>MGSSHHHHHHMIRKVLVANRGEIAVRIIRACQELGIRTVVAYSTADRDSLAVRLADEAVCIGPPPAAKSYLNAPALISAALVSGCDAIHPGYGFLSENPYFAEMCADCKLTFIGPPPEPIRLMGDKAIGRETMRKAGVPTVPGSDGEVRSLEEAIDVARQIGYPVLLKPSGGGGGRGMRVAYDEADLQRAFPTARAEAEAAFGNGALLLEKYLTRVRHVEIQVLADQYGHAIHLGERDCSAQRRHQKIVEEAPSPAVTPELRERMGADAVRGIKSIGYVNAGTLEFLLDQDGNYYFIEMNTRIQVEHPVTEQVTGIDLVRWQLLIASGERLTLRQEDIKITRHAIECRINAEDPERDFLPASGEVEFYLPPGGPGVRVDSHLYSGYTPPGTYDSLLAKIITFGDTRDEALNRMRRALNECVITGIKTTIPFQLALIDDPEFRAGRIHTGYVAELLRQWKETLNPV[2x]

Acetyl-CoA carboxylases (ACCs) convert acetyl-CoA to malonyl-CoA, a key step in fatty acid biosynthesis and autotrophic carbon fixation pathways. Three functionally distinct components, biotin carboxylase (BC), biotin carboxyl carrier protein (BCCP), and carboxyltransferase (CT), are either separated or partially fused in different combinations, forming heteromeric ACCs. Here, we identify two BC isoforms (BC1 and BC2) from Chloroflexus aurantiacus, a filamentous anoxygenic phototroph that employs 3-hydroxypropionate (3-HP) bi-cycle rather than Calvin cycle for autotrophic carbon fixation. To investigate the structural basis of BC1 as a bi-functional enzyme, we determined the crystal structures of BC1 and BC2 at 3.2 Å and 3.0 Å resolutions, respectively.

Notably, C. aurantiacus BC1 but not BC2, as well as the BCs from S. coelicolor, Roseiflexus castenholzii, and M. tuberculosis possess a C-terminal biotin/lipoyl attachment domain. Crystal packing analyses revealed two BC1 homodimers, but only one BC2 homodimer in each asymmetric unit. The superposition of one BC1-BC monomer with that of BC2 gave a root mean square deviation (RMSD) value of 0.654 Å, indicating that BC1 and BC2 possessed the same BC architectures. Each BC1-BC and BC2 homodimer was stabilized by extensive hydrogen bonding interactions between conserved amino acid pairs in the N- and C-terminal sub-domains. Specifically, the dimer interface residues Tyr44, Val328, Ser393 in BC1-BC homodimer, and Arg310 in BC2 dimer are not conserved with other reported BCs. Using NaHCO3 and biotin as substrates, both BC1 and BC2 were enzymatically active in catalyzing the biotin carboxylation reactions. However, BC1 had a relatively higher substrate affinity and turnover number than BC2. For BC2 that lacks a fused BCCP domain, it showed relatively lower biotin carboxylase activity and a dimer formation in solution. By contrast, the expression level of BC2 gradually decreases during the transition from respiratory to phototrophic conditions, suggesting that BC2 likely functions in pathways other than the 3-HP cycle. Since BC2 lacks the fused BCCP domain, it is probable that the BC2 participated biotin carboxylase reaction requires the involvement of a separate BCCP subunit (NCBI protein ID: ABY36917.1).>[4x]ILDTKPIPTIVDATTLGISGNTSGDYWLPTTMSLYQKELTDQIVSLHYSDILRYFETSHYKEDVILESMKTMCLNGSLVATHPYLLIDHYMPKSLITRDVPAHLAENSGKFSVLRDLINLVQEYETETAIVCRPGRTMDLLEALLLGNKVHIKRYDGHSIKSAAAANDFSCTVHLFSSEGINFTKYPIKSKARFDMLICLDTTVDTSQKDIQYLLQYKRERKGLERYA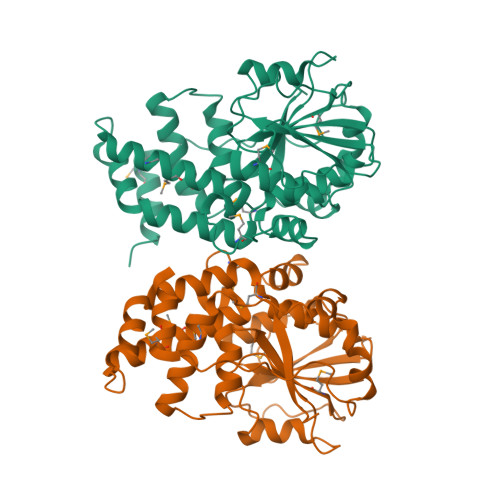PIVRLVAINSIDHCRLFFGKKFDKNSREYLENVTAAMVILRDRLGTLPPDLRPIYSQKLHYLVEWLENPTVPWPLPDIYPLKQYTSMDVERSLLTEVHFK Cilia and flagella-associated protein 410 (CFAP410) localizes at the basal body of cilia/flagella and plays essential roles in ciliogenesis, neuronal development and DNA damage repair. CFAP410 is a bimodular protein comprising two folded domains, i.e. NTD and CTD, which are connected through a variable unstructured loop. All these three crystal structures show a similar homotetrameric arrangement, with each monomer consisting of two α helices that form an open nutcracker-like conformation. Two CTDs first form an intercalated homodimer, and two such dimers further assemble into a tetramer by packing head-to-head through their first helices.

The CTD truncations that finally generated well-diffracting crystals were fragments covering residues 256–295, 212–246 and 213–246 of H. sapiens, T. brucei and C. reinhardtii CFAP410 proteins, respectively. However, those of TbCFAP410 and CrCFAP410 only partially dissolved in the buffer. We, therefore, carried out refolding for the insoluble polypeptides using the following protocol. The final condition for crystallizing the TbCFAP410-CTD contained 2.0 M (NH4)2SO4 and 5% (v/v) iso-propanol (4°C). The crystal structure of TbCFAP410-CTD was determined de novo using ARCIMBOLDO. Our in vivo data showed that TbCFAP410 localizes to both the basal body and the posterior cell tip. We observed that the A267E mutant that breaks the tetramer into two dimers could still localize to the posterior cell tip, but failed to target to the basal body. However, the disease-causing mutant L272P of TbCFAP410 completely lost its localization to both the posterior cell tip and the basal body. It suggests that targeting TbCFAP410 to the basal body requires the tetrameric assembly of the CTD. Therefore, we conclude that the localization of TbCFAP410 to the basal body and the posterior cell tip requires the CTD and its ability to oligomerize.

>[2x]QIGPTETGVVQAVKVLLSELSVEGLDEVRRFIDALQ>[2x]MSVERGTSNSASYKMFLTHGGSPISYFHDVPLFADATNNCYNMIVEIPRWTNAKMEICKEE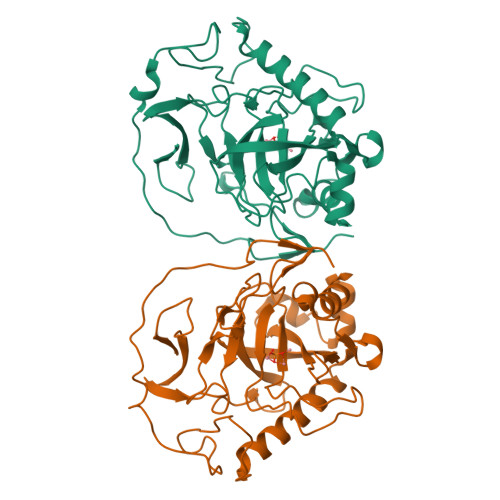LMNPIKHDVKNNKLRYIYNVFPHKGYIWNYGALPQTWEDPSYVDEDTKAKGDNDPIDVCEIGSKIWPSGSVIPVKVLGILGMIDEGETDWKVIAINVADPMAEKLNDILDVDAHMPGFLKATRDWFKYYKVPAGKPENSFAFNGEFKNKEFAAKIISKTHEHWQKLISTKVEAGPIIRANVTVKGSPYMVSKEDFIDALQKHEDFKRGSEPTDQAIEQWHFCNTNI>MSTVPELLARQVTRAPDAVAVVDRDRVLTYRELDELAGRLSGRLIGRGVRRGDRVAVLLDRSADLVVTLLAIWKAGAAYVPVDAGYPAPRVAFMVADSGASRMVCSAATRDGVPEGIEAIVVTDEEAFEASAAGARPGDLAYVMYTSGSTGIPKGVAVPHRSVAELAGNPGWAVEPGDAVLMHAPYAFDASLFEIWVPLVSGGRVVIAEPGPVDARRLREAISSGVTRAYLTAGSFRAVAEESPESFAGLREVLTGGDVVPAHAVARVRSACPRVRIRHMYGPTETTMCATWHLLEPGDEIGPVLPIGRPLPGRRAQVLDASLRAVAPGVIGDLYLSGAGLADGYLRRAGLTAERFVADPSAPGARMYRTGDLAQWTADGALLFAGRADDQGSHHHHHH[2x];>[2x]MTNPFDNEDGSFLVLVNGEGQHSLWPAFAEVPDGWTGVHGPASRQDCLGYVEQNWTDLRPKSLISQISD

In this work, we have sought to understand the evolutionary history of lipid II targeting glycopeptide antibiotics (GPAs), a vital class of nonribosomal peptides used in the clinic for the treatment of resistant bacterial infections and exemplified by vancomycin (Van) and teicoplanin (Tei). Since ANC1-3 domains display polydisperse elution profiles in size exclusion chromatography, we instead turned to the characterisation of an Acore construct of the Hpg accepting A1 domain from Tei biosynthesis (A1tei), which possesses a homologous pocket to ANC1. The MbtH-like domain Tcp13 also exhibits the anticipated fold, containing a 3-stranded antiparallel β-sheet and an α-helix adjoining the centre of the sheet.

To understand the effects of the evolutionary mutations seen in the binding pocket of the ANC A-domains we then mutated the residues of the substrate binding pocket of A1tei to those seen in A1ANC2 and A1ANC3. Comparing the A1ANC3 pocket to A1ANC2 shows further refinement of the pocket through additional substitutions (L287M and V295M), which serve to improve van der Waals contacts in the binding pocket for Leu. ANC2 and ANC3 were both selective for Leu, with ANC3 showing 1.7-/3.8 fold higher kcat value for L-Leu/D-Leu. In terms of A1-domain evolution, our results indicate how the alteration of the Hpg binding pocket was driven through three crucial changes in the binding pocket that together eliminated Hpg binding whilst enabling the acceptance of Leu.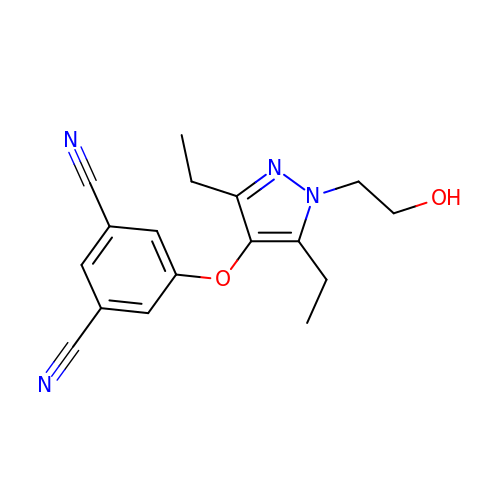5-{[3,5-diethyl-1-(2-hydroxyethyl)-1H-pyrazol-4-yl]oxy}benzene-1,3-dicarbonitrile  | C17 H18 N4 O2 | MCPUZZJBAHRIPO-UHFFFAOYSA-N> EPEWTYP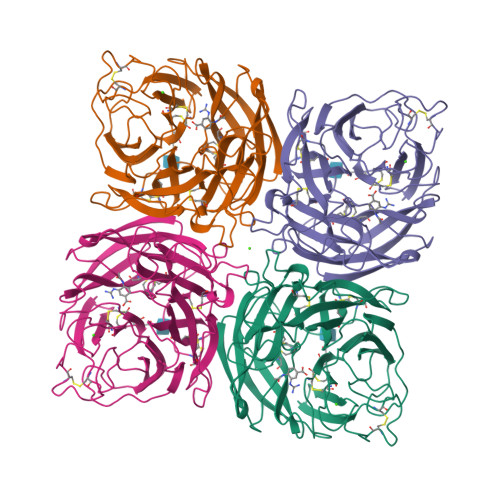RLSCQGSTFQKALLISPHRFGEIKGNSAPLIIREPFVACGPKECRHFALTHYAAQPGGYYNGTRKDRNKLRHLVSVKLGKIPTVENSIFHMAAWSGSACHDGREWTYIGVDGPDNDALVKIKYGEAYTDTYHSYAHNILRTQESACNCIGGDCYLMITDGSASGISKCRFLKIREGRIIKEILPTGRVEHTEECTCGFASNKTIECACRDNSYTAKRPFVKLNVETDTAEIRLMCTKTYLDTPRPDDGSIAGPCESNGDKWLGGIKGGFVHQRMASKIGRWYSRTMSKTNRMGMELYVKYDGDPWTDSDALTLSGVMVSIEEPGWYSFGFEIKDKKCDVPCIGIEMVHDGGKDTWHSAATAIYCLMGSGQLLWDTVTGVDMAL>[2x]GSFVEMVDNLRGKSGQGYYVEMTVGSPPQTLNILVDTGSSNFAVGAAPHPFLHRYYQRQLSSTYRDLRKGVYVPYTQGKWEGELGTDLVSIPHGPNVTVRANIAAITESDKFFINGSNWEGILGLAYAEIARP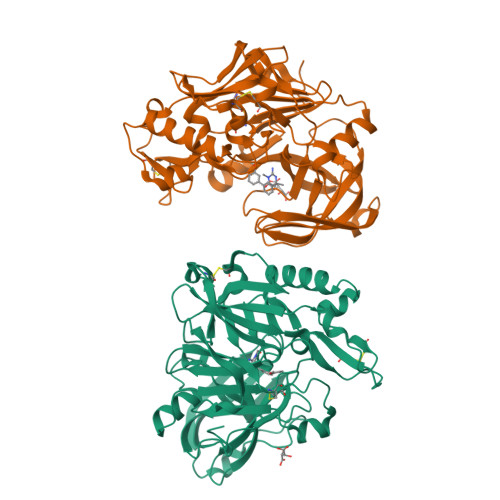DDSLEPFFDSLVKQTHVPNLFSLQLCGAGFPLNQSEVLASVGGSMIIGGIDHSLYTGSLWYTPIRREWYYEVIIVRVEINGQDLKMDCKEYNYDKSIVDSGTTNLRLPKKVFEAAVKSIKAASSTEKFPDGFWLGEQLVCWQAGTTPWNIFPVISLYLMGEVTNQSFRITILPQQYLRPVEDVATSQDDCYKFAISQSSTGTVMGAVIMEGFYVVFDRARKRIGFAVSACHVHDEFRTAAVEGPFVTLDMEDCGYNI2-[4-[(3'R,4S)-3'-fluoro-1-[2-[(4-fluorophenyl)methyl-[(1S)-2,2,2-trifluoro-1-methyl-ethyl]amino]-2-oxo-ethyl]-2,5-dioxo-spiro[imidazolidine-4,1'-indane]-5'-yl]pyrazol-1-yl]-N-methyl-acetamide 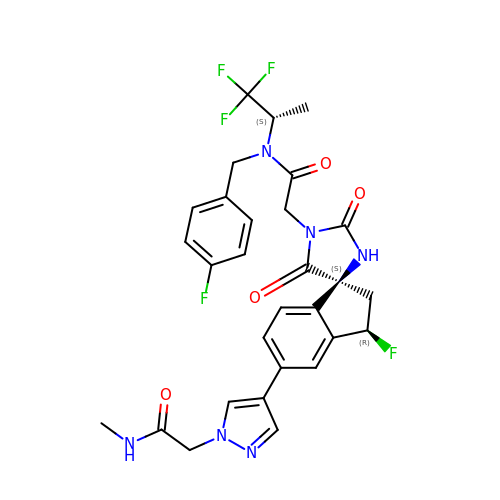| C29 H27 F5 N6 O4 | SWXCHCQCWFXILM-DAXQEMQKSA-N> CTGLALETKDGLHLFGLNMDIEYSFNQSIIFIPRNFKCVNKSNKKELTTKYAVLGMGTIFDDYPTFADGMNEKGLGCAGLNFPVYVSYSKEDIEGKTNIPVYNFLLWVLANFSSVEEVKE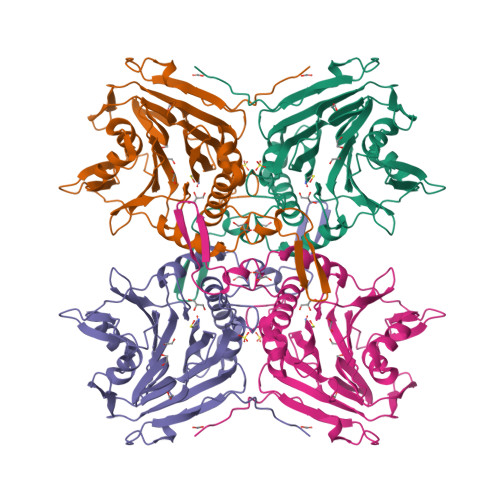ALKNANIVDIPISENIPNTTLHWMISDITGKSIVVEQTKEKLNVFDNNIGVLTNSPTFDWHVANLNQYVGLRYNQVPEFKLGDQSLTALGQGTGLVGLPGDFTPASRFIRVAFLRDAMIKNDKDSIDLIEFFHILNNVAMVRGSTRTVEEKSDLTQYTSCMCLEKGIYYYNTYENNQINAIDMNKENLDGNEIKTYKYNKTLSINHVN>[3x]SNAMLKYQQIATEIETYIEEHQLQQGDKLPVL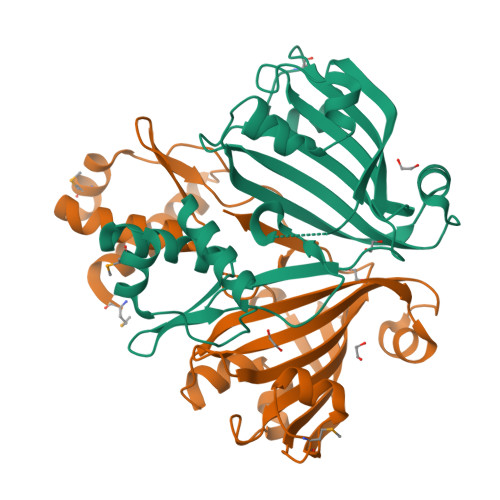ETLMAQFEVSKSTITKSLELLEQKGAIFQVRGSGIFVRKHKRKGYISLLSNQGFKKDLEDFNVTSKVIELDVRKPTPEAAENLNIGMDEDIYYVKRVRYINGQTLCYEESYYTKSIVTYLNNEIVSHSIFHYIREGLGLKIGFSDLFLHVGQLNEEEAEYLGLEAGLPKLYIESIFHLTNGQPFDYSKISYNYEQSQFVVQANSFLL> MGESERSEAFGIPRDSPLSSGDAAELEQLRREAAVLREQLENAVGSHAPTRSARDIHQLEARIDSLAARNSKLMETLKEARQQLLALREEVDRLGQPPSGYGVLLATHDD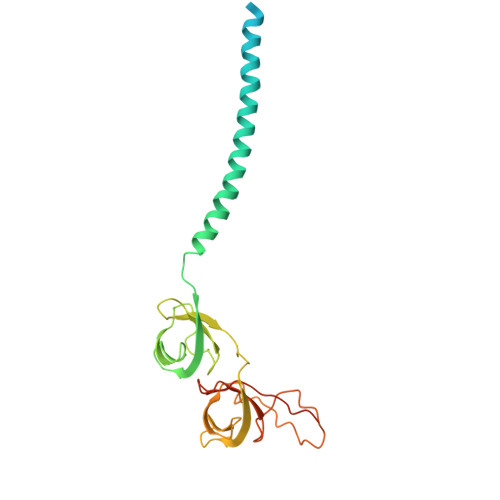DTVDVFTSGRKMRLTCSPNIDAASLKKGQTVRLNEALTVVEAGTFEAVGEISTLREILADGHRALVVGHADEERVVWLADPLIAEDLPDGLPEALNDDTRPRKLRPGDSLLVDTKAGYAFERIPLVPRGSAAALEHHHHHH>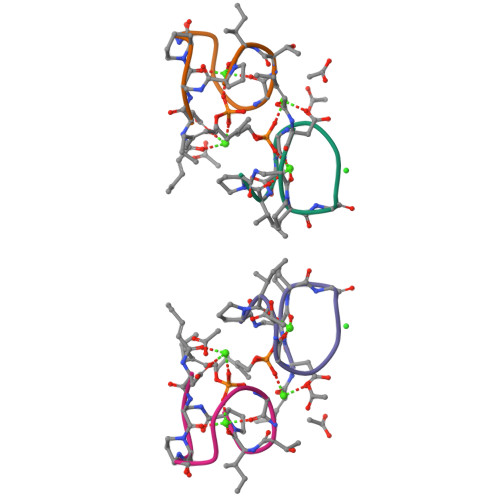XDAXGDGDGTIP[2x]2-deoxy-alpha-D-galactopyranose 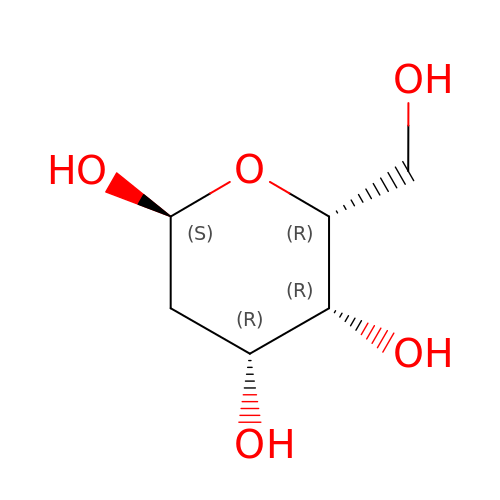| C6 H12 O5 | PMMURAAUARKVCB-ARQDHWQXSA-N>[2x]GGAACUAGCUCAGCAUA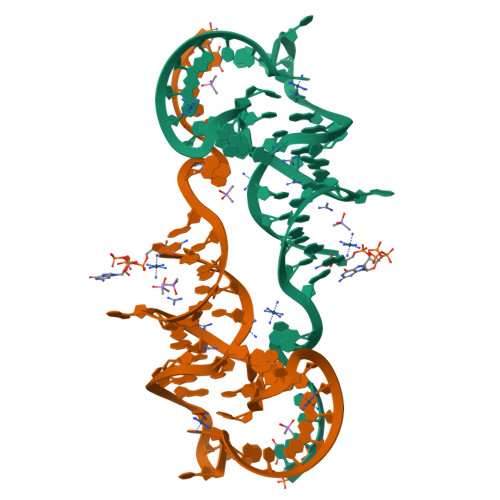CACGAGUUGCAAGCAUGGGAAGUUCAAGCCUCGU>SANFTDKNGRQSKGVLLLRTLAMPSDTNANGDIFGGWIMSQMDMGGAILAKEIAHGRVVTVAVESMNFIKPISVGDVVCCYGQCLKVGRSSIKIKVEVWVKKVASEPIGERYCVTDAVFTFVAVDNNGRSRTIPRENNQEL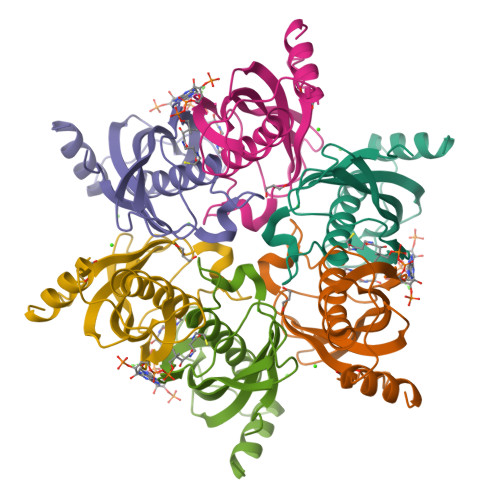EKALALISEQPL[2x]> TTPQEDGFLRLKIASKEKIARDIWSFELTDPQGAPLPPFEAGANLTVAVPNGSRRTYSLCNDSQERNRYVIAVKRDSNGRGGSISFIDDTSEGDAVEVSLPRNEFPLDKRAKSFILVAGGIGITPMLSMARQLRAEGLRSFRLYYLTRDP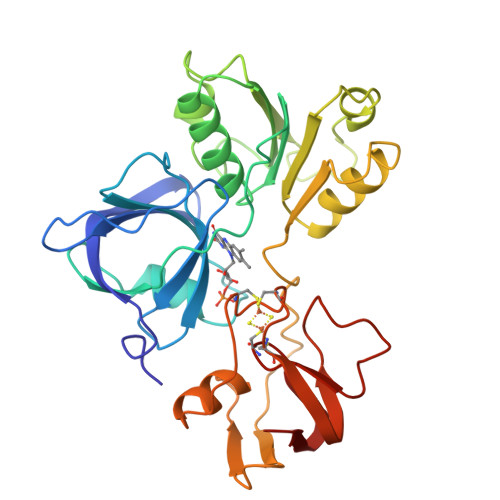EGTAFFDELTSDEWRSDVKIHHDHGDPTKAFDFWSVFEKSKPAQHVYCCGPQALMDTVRDMTGHWPSGTVHFESFGATNTNARENTPFTVRLSRSGTSFEIPANRSILEVLRDANVRVPSSCESGTCGSCKTALCSGEADHRDMVLRDDEKGTQIMVCVSRAKSAELVLDL>MSRVLLCSAGHSSMVVPEAFHAVPEGFEEVHVFTTDSEKFNPVVLNDFFHSLPNVRFSITKCHGLADILNERDFEFYQEMLWQWYLTKMPDNELPYVCLSGGIKSMSASLQKAATLFGAQS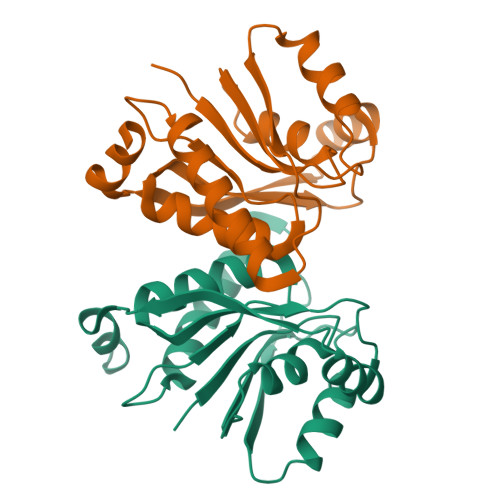VFHVLADNNPRNIEEMFDALQKGQIHFIEMGYEPGWAALRRLKKI[4x]9H-xanthene-1,3,6,8-tetrol | 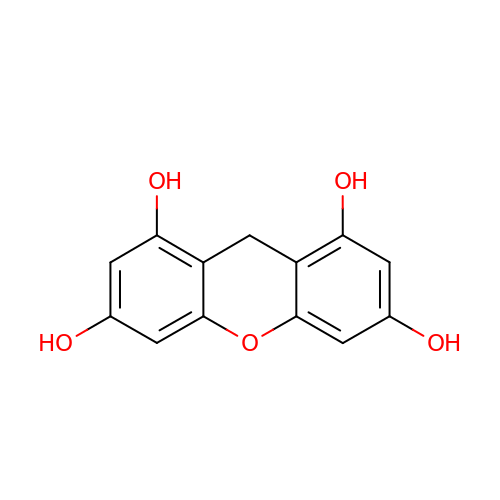C13 H10 O5 | WRWDLBILCDUPOS-UHFFFAOYSA-N>DNPLESPPPEIVKQGKEAVRQYFQSIEEARSKGEALVHLQEIKVHLIGDGMAGKTSLLKQLIGETFDPKESQTHGLNVVTKQAPNIKGLENDDELKECLFHFWDFGGQEIMHASHQFFMTRSSVYMLLLDSRTDSNKHYWLRHIEKYGGKSPVIVVMNKIDENPSYNIEQKKINERFPAIENRFHRISCKNGDGVESIAKSLKSAVLHPDSIYGTPLAPSWIKVKEKLVEATTAQRYLNRTEVEKICNDSGITDPGERKTLLGYLNNLGIVLYFEALDLSEIYVLDPHWVTIGVYRIINSSK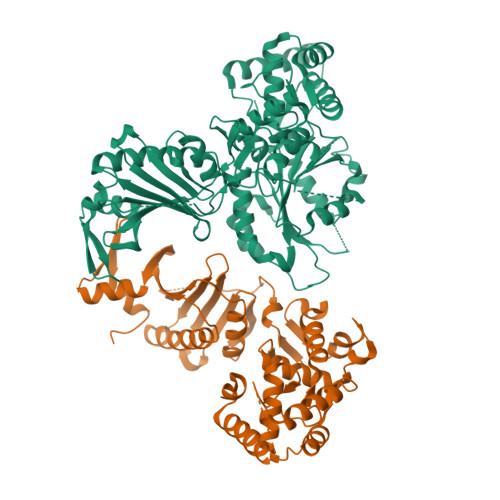TKNGHLNTSALGYILNEEQIRCDEYDPAKNNKFTYTLLEQRYLLDIMKQFELCYDEGKGLFIIPSNLPTQIDNEPEITEGEPLRFIMKYDYLPSTIIPRLMIAMQHQILDRMQWRYGMVLKSQDHEGALAKVVAETKDSTITIAIQGEPRCKREYLSIIWYEIKKINANFTNLDVKEFIPLPGHPDELVEYKELLGLEKMGRDRYVSGKLEKVFSVSKMLDSVISKEERNKER[2x]> MNKESKDDDMSLGKFSFSHFLYYLVLIVVIVYGLYKLFTGHGSDINFGKFLLRTSPYMWANLGIALCVGLSVVGAAWGIFITGSSMIGAGVRAPRITTKNLISIIFCEVVAIYGLIIAIVFS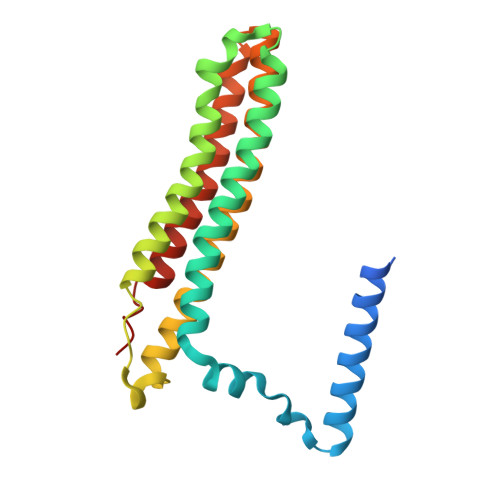SKLTVATAENMYSKSNLYTGYSLFWAGITVGASNLICGIAVGITGATAAISDAADSALFVKILVIEIFGSILGLLGLIVGLLMAGKASEFQ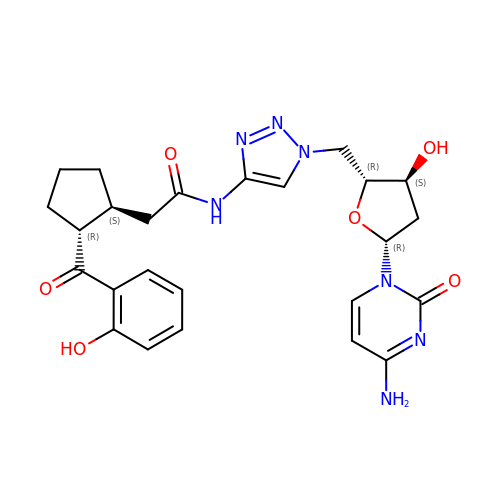2',5'-dideoxy-5'-[4-({[(1S,2R)-2-(2-hydroxybenzene-1-carbonyl)cyclopentyl]acetyl}amino)-1H-1,2,3-triazol-1-yl]cytidine | C25 H29 N7 O6 | QYQWONZWXIVWAC-CBSYKJJGSA-N> MKQILDSARNYLKNNSRIKTASLISLELPGSTGTSTAFIYLTDYFRDVIYNGILYQAGKVKSISPHKQNRDLSIGSLSFTITGTAQDEVLKLVQNGVSFLDRTVSIHQAIITEDGSILPVDPDTNGPLLYFRGRITGGGIKDNISTSGVGTSTITWNCSNQFYDFDRVNGRYTDDASHRGLEVVAGQLLPSNGAKRLEYQEDYGFFHANKSISILAKYQVQEERYKLKSKKKLFGLSRSYSLKKYYETVTKEVDIDFNLAAKYIPVVYGVQKIPGIPIFADTELHNPNIVYVVYAFAEGEIDGFLDFSFGDNPMICVDANDSSARTCFGTKKIVGDTMQRIASGISSSSPSVHGQEYRYNDGNGDIRIWTYHGKSNQTASDVLVNIARNRGFYLQNMNGNGPEYWDARYKLLDTAYAVVRFTINENRTEIPEVSAEIQGKKVKVYHSDGRVTANSTSLNGIWQTLDYLTSDRYGANITIDQFPLQQLIQEAAILDIIDESYQVSWQPYWRYVGWTNPLAENRQIVQMNTILDTSESVFKNVQGLLESYGGAINNLSGQYRVTVEKYSNTPLEINFLDTYGDLELSDTTGRNKFNSVQASIVDPALSWKTNSITFYNSNYKEQDKNLDKKLQLSFANITNYYTARSFADRELKKSRYSRTLSFSLPYQFIGIEPNDAIAFTYDRYGWDRKYFLVDEVENSREGKINVTLQEYGEDVFINSGQVDNSGNDIPDISNNVLPPRDFKYTPTPGGLVGSIGKNGELSWLPSLTNNVVYYSIVHSGHAEPYIVQQLETNPNERMIQEIIGEPAGLAIFEIRAVDINGRRSSPVTLSIELNSAKNLSVVSNFRVTNTASGDVTEFVGPDVKLAWDRIPEEDIIESIFYTLEIHDPQNRMLRSVRIENQYTYDYLLTYNKADFALQNSDALGINRKLYFRIRAEGDDGEQSVEWASI;>MRLPDPYTNPELSGLGFESVNLIDNDPVIRDELPNGKVNEVKVSAQYWGINISYPELFPDEYSVLDAFILEYKRTGGYIDVILPQYEAFRVRGNTNLVNIPAGQKGSNITMDTQGVLTGIPKPGDLFKLSNHPKVYKITSFNRSGNSWSINVYPDLFITTTGAEKPVFNGILFRTKLMNGDAFGSTLNNNGTYSGISLNLRESL[2x];> MYYSLMRESKVIVEYDGRAFHFDALSNYDVQTSYEEFKTLRRTIHRRTNYADSVINAQTPSSISLAINFSNTLTEANFFEWLGFDRKGNTFLLPLYSNNIEPIMFNIYIVNKDNNCVYFENCYVSTVDFSLDKNIPILNVGIESGKFSEVSTYREAASIIQGEAMSYSPVIVSTNGNILPGLISASLSFQQQCSWREDKSVFDINKIYNNKRAYVNEMNASATISLYYLKRFAGDMVYNIEPETDVPLNIRNNNISIDFPLARISKRLNFSDVYKVEWDIIPTASSDPVRIDFFGEIKND;>MSTENRVIDIVVDEKVPYGLIMQFMDVDDSVYPPSEIPVNLTGYSLRGTIKSSLDENAETLASFTTSIIDAAQGAAAISLSVADVTNIGEKASKERDKYNPRQRFAGYYDILMTRDVIGSEVSSFRIMEGKVYISDGVTQ[4x];>MALKTKIIVQQILNIDDTTTTASKYPKYTVVLGNSISSITAGELTAAVEASAGSAAAAKGSEIAAKESELNAKDSENEAAISAGASEESASQSAASAAESERQAGLSKGSADNSAASAQESEGFRDSAELAAQNAEQSRLLAEQAKTAAQQAQTAAEAAKTGAETAKDGADAAATTAGEHAAAARQSELNAKISETNAAGSATEAGDKAIDATTEADRAKAEADRATQIVDSKLDKVDISGFIKVYKTKAEADADVVNRVLDEKVLVWNQTNSKYGWYKVAGTAETPVLELVETEQKLTSVNNVRADDAGNVQITLPGGNPSLWLGEVTWFPYDKDSGVGYPGVLPADGREVLRVDYPDTWEAIEAGLIPSVSEAEWQAGASLYFSTGDGSTTFRLPDMMQGQAFRAPTKGEEDAGVIKDQIPYVVTVNGISPDAITGNVEIDTSLQGTVSINQGGTGATTKEDARIALELYSTTEVDSALADKADIATTYTKTEVDSALADKADIATTYTKVEVDSALADAKTQSDTDYLLKANNLSDLADRAAAWLNVRPIGSTPLAGDPVGDYDAVTKRWVENKINTGTVGPTMNGVMNYGVGDFHLRDSRAYIQPYEVVSDGQLLNRADWPELWAYAQMLSPISDADWLADPTKRGQYSLGDGSTTFRVPDRNGVQTGSISALFGRGDGGASSTGGTILDSAAPNITGSFGRLVYASTGTIYEANTGTGAFSAVLSQAKYKRLSEISAADGTAATYPSGFEFFASNSSPVYGRGSTEVRPKAFTGVWVIRASGGFVAANTSWSVINGDATRPADGTTADGGEIISRYNVNGVREAQMSWRIRAQIGAEHYARLNVYNATANRTAVYDFNDLGTFSAENLHSKGAIYSDGNLTIQNQGWPGINFKSNRYNTPATQIGGSTIIEVSGTDGNVSGVNLIRRRGDGNQAGQIIVSFPTTGGAIALQGTSGIEYKKDVTDADAQEAMDRINGQRLVNFVYKDDEQERVRFGVIAEEAELIAPQYIKHNQVSYEDILDEEGNKIGEKTRDRPSVDVNPIVMDLMGCVQALNAKIAALEARIAELESKE[3x];> MTDKLIRELLIDVKQKGATRTAKSIENVSDALENAAAASELTNEQLGKMPKTLYSIERAADRAAKSLTKMQASRGMAGITKSIDSIGAKLDDLSIAMIEVADKLEAGFDGVSRSVKVMGNDVAAATEKVQDRLYDTNRVLGGTARGFNDTAGAAGRASRAIGNTSGSARGATRDFAAMAKVGGGLPLLYAAIASNIFVLQSAFEQLKLGDQLNRLEEFGVIVGTQTGTPVQSLARSLQEAAGYAISFEEAMRQASSASAYGFDAEQLNKFGLVARRAAAVLGVDMTDALNRVIKGVSKQEIELLDELGVTIRLNDAYADYVKQLNAANTGITYNINSLTTFQKQQAYANAVIAESTKRFGYLDEVLRATPWEQFAANADAALRTIQQAAAKYLGPVIDAINTVFYTSQASISAEAARAQEQTNKQIDPTNVGAVALSLSASEEGYNKALDMYKESLDKRNKLKSEFDKRMEQADFYTKLAIRQVGEGIPAGLATAGASEANKKFVEETAAMGLQVARLDKEVTDSTENLNAWKSAYQAAGAAAAKANPEFQKQINLQRDTTDPGAVYDFNSTVLKGLTEQQKAYNQTKKTASDLANDIQNVAQNTDTAAKTSATLADAIKNIESLSLGTGKSADEYVKNLNLGYNTLSEMKTASQALSEYVKLTGNETKNQLAVQQKIADVYNQTKDKEKAQEAGRRLELQQLEEQEAALRRVLQTNQGNKAVEREIEKIQLEKIKLTNQGMEAQKKVKDYTDKILGVDREIALLNNRTMTDTQYRLAQLNLELTIEKEKYEWYTKQADKQKEAEQSRRAQAQIEREIWKFHQDQQAEMTSKRQEAFENTLTSMFPLAGEMQKMEMQLDFYTQMKELTKDNANEQMRWNAEIAKTRAQMSALTAQRNAQMQSSVGSSLGAVYTPTTGLSGEDKKFADMGNQLASYDQAISKLSELNSEATAVAQSMGNLANAMIQFSQGSLDTTSTIAVGMQTVASMIQYSTSQQVSAIDQAIAAEQKRDGKSEASKAKLKKLEAEKLKIQQDAAKKQIIIQTAVAVMQAATAVPYPFSIPLMIAAGLAGALALAQASSASGMSSIGDSGADTASYLTLGERQKNIDVSMSANAGELSYVRGDKGIGNANSFVPRAEGGNMYPGVSYQMGEHGTEVVTPMVPMKATPNDELKNSSNSTAGRPIILNISAMDAASFREFASSNSGALRDAVELALNENGASLKTLGNS;> MSLQLLRNTRIFVSTVKTGHDTTNTQEILVQDDISWGQDSNSTDITVNEAGPRPTRGSKRFNDSLNAAEWSFSTYILPYEDTTTGKQIVPDYMLWHALSSGKAIDLDGDTGAHNNATNFMVNFKDNAYHELAMLHIYILTDNAWSYIDSCQINQAEVNVDIEDIGRVTWSGNGNQLIPLDEQPFDPDALGIDDETYMTIQSSYIKNKLTILKIKDMDSDKEYDIPITGGTFTINNNITYLTPNIMSRVNIPIGSFTGAFELTGSLTAYLNDKSLGSMELYKDLVRTLKVVNRFEIALILGGEYDDERPAAVLVAKQAHVNIPTIETDDVLGTSVEFKAIPTDLDTGDEGYLGFSNKYTKTTVANLIATGDGAETPPILVESITVKSAADATSVTNSDTLQMSVEVTPPEATNTAVTWSISSGDAATIDAESGLLTADVSKTGEVIVKAVAKDGSGVEGTKTITVSAGE

The T5 family of viruses are tailed bacteriophages characterized by a long non-contractile tail. The bacteriophage DT57C is closely related to the paradigmal T5 phage, though it recognizes a different receptor (BtuB) and features highly divergent lateral tail fibers (LTF). We present a composite map determined by electron cryo-microscopy (cryo-EM) at resolutions ranging between 2.9 Å to 4.9 Å of the entire T5-like phage particle DT57C, and atomic models comprising its core structural proteins. Our results provide a complete atomic structure of a T5-like phage, provide insights into the process of DNA ejection as well as a structural basis for the design of engineered phages and future mechanistic studies.

The first layer directly interacts with the last TTP ring and is composed of an inner trimeric ring of TTMP surrounded by a dodecameric ring of LtfC. The inner trimeric TTMP ring is surrounded by an outer ring composed of 12 LtfC monomers. LtfC adopts a compact, single-domain structure composed mostly of β-sheets, with each TTMP monomer contacted by four copies of LtfC. A cavity remains between the TTMP and the part of the LtfC ring distal to the tail tube, into which LtfA is inserted. The N-terminal portions of LtfA form a lasso-like structure filling the groove between the LtfC and TTMP rings, such that each LtfA copy extends in opposite direction as observed from the outer end of the helical bundle. The capsid-distal LtfA contacts the capsid-proximal LtfA from an adjacent LtfA trimer, enabling the formation of a closed ring. The β-strands of all LtfA copies interact with the LtfC ring by augmenting their β-sheets of the latter to eight- or nine-stranded sheets by donating one or two strands from LtfA. The loops of the two long β-hairpins of TTMP extend tailward and contact the next ring, composed of six copies of Dit. Finally, a trimer of TTHP closes the tail tip complex. The cavity enclosed by the TTHP also contained additional density for a small α-helical coiled coil region, which was assigned as the C-terminal part of the TMP based on its location within the lumen of the tail tube tip, the fact that this region is predicted α-helical, and a close fit to the AlphaFold model.> VDMSNVVKTYDLQDGSKVHVFKDGKMGMENKFGKSMNMPEGKVM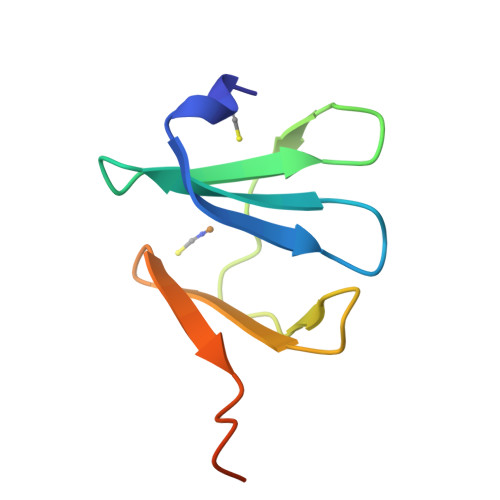ETRDGTKIIMKGNEIFRLDEALRKGHSEGG> GPGSADEEQVFHFYWLDAYEDQYNQPGVVFLFGKVWIESAETHVSCCVMVKNIERTLYFLPREMKIDLNTGKETGTPISMKDVYEEFDEKIATKYKIMKFKSKPVEKNYAFEIPDVPEKSEYLEVKYSAEMPQLPQDLKGETFSHVFGTNTSSLELFLMNRKIKGPCWLEVKSPQLLNQPVSWCKVEAMALKPDLVNVIKDVSPPPLVVMAFSMKTMQNAKNHQNEIIAMAALVHHSFALDKAAPKPPFQSHFCVVSKPKDCIFPYAFKEVIEKKNVKVEVAATERTLLGFFLAKVHKIDPDIIVGHNIYGFELEVLLQRINVCKAPHWSKIGRLKRSNMPKLGGRSGFGERNATCGRMICDVEISAKELIRCKSYHLSELVQQILKTERVVIPMENIQNMYSESSQLLYLLEHTWKDAKFILQIMCELNVLPLALQITNIAGNIMSRTLMGGRSERNEFLLLHAFYENNYIVPDKQIFRKPQQKLGDEDEEIDGDTNKYKKGRKKAAYAGGLVLDPKVGFYDKFILLLDFNSLYPSIIQEFNICFTTVQRVASEAQKVTEDGEQEQIPELPDPSLEMGILPREIRKLVERRKQVKQLMKQQDLNPDLILQYDIRQKALKLTANSMYGCLGFSYSRFYAKPLAALVTYKGREILMHTKEMVQKMNLEVIYGDTDSIMINTNSTNLEEVFKLGNKVKSEVNKLYKLLEIDIDGVFKSLLLLKKKKYAALVVEPTSDGNYVTKQELKGLDIVRRDWCDLAKDTGNFVIGQILSDQSRDTIVENIQKRLIEIGENVLNGSVPVSQFEINKALTKDPQDYPDKKSLPHVHVALWINSQGGRKVKAGDTVSYVICQDGSNLTASQRAYAPEQLQKQDNLTIDTQYYLAQQIHPVVARICEPIDGIDAVLIATWLGLDPTQFRVHHYHKDEENDALLGGPAQLTDEEKYRDCERFKCPCPTCGTENIYDNVFDGSGTDMEPSLYRCSNIDCKASPLTFTVQLSNKLIMDIRRFIKKYYDGWLICEEPTCRNRTRHLPLQFSRTGPLCPACMKATLQPEYSDKSLYTQLCFYRYIFDAECALEKLTTDHEKDKLK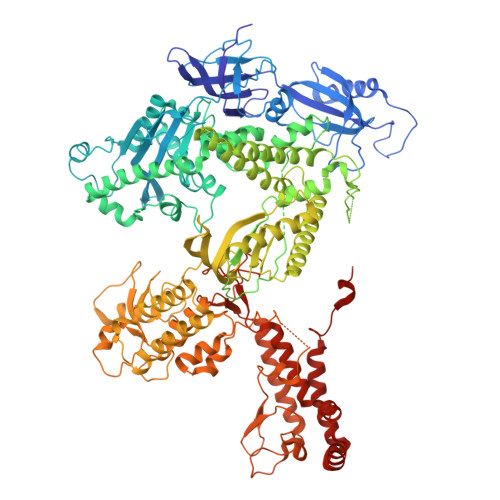KQFFTPKVLQDYRKLKNTAEQFLSRSGYSEVNLSKLFAGCAVKS> MNVIAILNHMGVYFKEEPIRELHRALERLNFQIVYPNDRDDLLKLIENNARLCGVIFDWDKYNLELCEEISKMNENLPLYAFANTYSTLDVSLNDLRLQISFFEYALGAAEDIANKIKQTTDEYINTILPPLTKALFKYVREGKYTFCTPGHMGGTAFQKSPVGSLFYDFFGPNTMKSDISISVSELGSLLDHSGPHKEAEQYIARVFNADRSYMVTNGTSTANKIVGMYSAPAGSTILIDRNCHKSLTHLMMMSDVTPIYFRPTRNAYGILGGIPQSEFQHATIAKRVKETPNATWPVHAVITNSTYDGLLYNTDFIKKTLDVKSIHFDSAWVPYTNFSPIYEGKCGMSGGRVEGKVIYETQSTHKLLAAFSQASMIHVKGDVNEETFNEAYMMHTTTSPHYGIVASTETAAAMMKGNAGKRLINGSIERAIKFRKEIKRLRTESDGWFFDVWQPDHIDTTECWPLRSDSTWHGFKNIDNEHMYLDPIKVTLLTPGMEKDGTMSDFGIPASIVAKYLDEHGIVVEKTGPYNLLFLFSIGIDKTKALSLLRALTDFKRAFDLNLRVKNMLPSLYREDPEFYENMRIQELAQNIHKLIVHHNLPDLMYRAFEVLPTMVMTPYAAFQKELHGMTEEVYLDEMVGRINANMILPYPPGVPLVMPGEMITEESRPVLEFLQMLCEIGAHYPGFETDIHGAYRQADGRYTVKVLKE

extracellular pH, and works in conjunction with a cognate inner membrane antiporter. excreted by the antiporter in exchange for a new amino acid substrate. that it is a decamer made of two pentameric rings. central pore, with the CTDs at the periphery.

the LdcI at active pH (LdcIa, pH 6.2). 7.5 Å to 6.2 Å resolution. whole upon enzyme activation by pH and the binding of LARA. decameric state upon activation and incorporation into the LdcI-RavA cage.>MNHKVHHHHHHIEGRHMELNPPEIVRHIV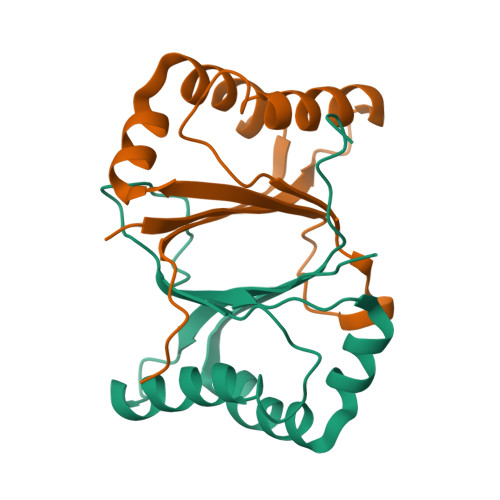FNRYKSQLSQKQIDQIIADYGNLQNIAPEMKEWKWGTDLGPAVEDRADGFTHAYESTFHSVADFLNFFYSPPALEFAKEFFPACEKIVVLNYIINETFPYTWALPNKYVVT[12x]> MASLPKRIIKETEKLVSDPVPGITAEPHDDNLRYFQVTIEGPEQSPYEDGIFELELYLPDDYPMEAPKVRFLTKIYHPNIDRLGRICLDVLKTNWSPALQIRTVLLSIQALLASPNPNDPLANDVAEDWIKNEQGAKAK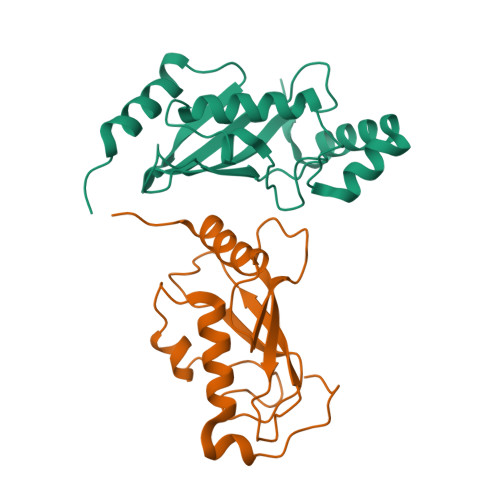AREWTKLYAKKKP;> MSKVPRNFRLLEELEKGEKGFGPESCSYGLADSDDITMTKWNGTILGPPHSNHENRIYSLSIDCGPNYPDSPPKVTFISKINLPCVNPTTGEVQTDFHTLRDWKRAYTMETLLLDLRKEMATPANKKLRQPKEGETF>[2x]MSLRMKVF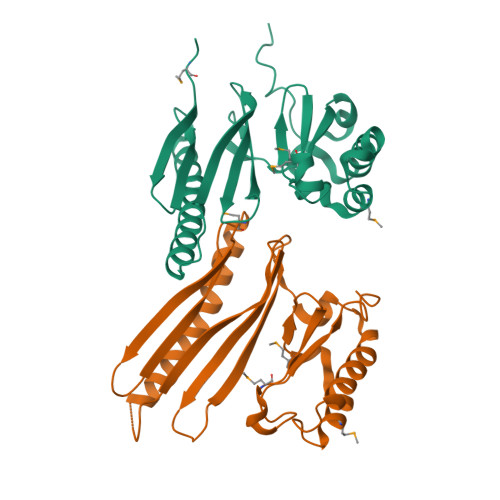EIVKSSTENEIVRIHVELPRLKYLKDSNFEEKFNSEVEEKIKKFVNEVKGIAQEDHDKDVQHTPYEAYVSVDVRYEGKDFLSFVVYYYQFTGGAHGITFFETYNIDLKNSKVLKLYDIIKEEAEDTIKSNILKQIEQNNTDFFPDAPMNILKDDIFSREFTISKDGLIIMYPHYDLAPYASGMPEFVIPWNVIEKFLKYDILSLLKEGHHHHHH> MDPLRAQQLAAELEVEMM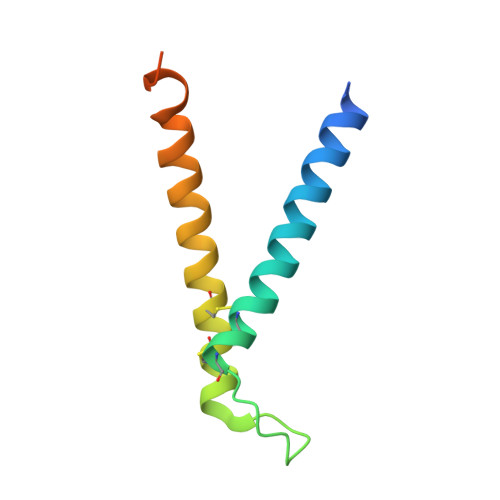ADMYNRMTSACHRKCVPPHYKEAELSKGESVCLDRCVSKYLDIHERMGKKLTELSMQDEELMKRVQQSSGPA> MTGIPTVTARPWTQRPRAENSTTNPTYFFTFGDSYSQTGFSASGTQPSASNPMGNPDLGIGTTTNGPNWIGYLTTTENASLVLSYNLAAGGATIDNALVPAYPGDLASQFRLFEDVYADKPASAPWSAEDAVFGVWIGINDIGNAYYSTDAETYTPKLISRLESLVEEVYKNGGRKFLFLNVPPTSRSPLFLEQGEEVVKQHAEYLSVYNENLEGMVDDFTKKKGDVTTVLYDSWSFMTKILDDPTAYGFPDATCINDDGTSCIWWDNWHP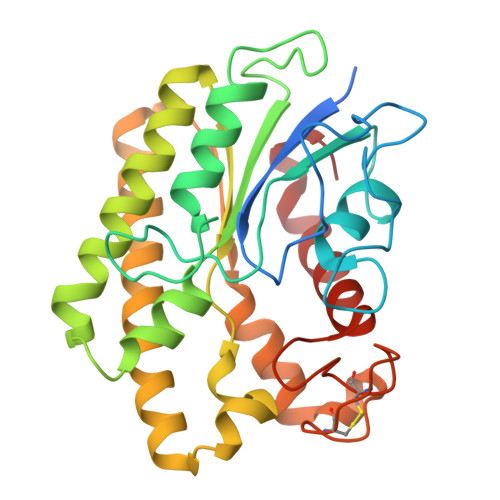GMKYHLLQAEDMKPKLRKLGGW>[2x]GSHMASMPKQLSSVTFHNGRKMPVVGLGTWQSPPEEVTAAIDVALEVGYRHIDTAFMYQNEAAIGKTLKKWFDSGKLKREDVFIVTKLPPIGNRAESVEKFLTKSLEALQLDYVDLYLIHLPVGFQYKGDDNLWPRGEAGEFLIDTSTDLISLWKAMEAQVDAGRTRSVGLSNFNSRQIARIVKSARIRPANLQVELNV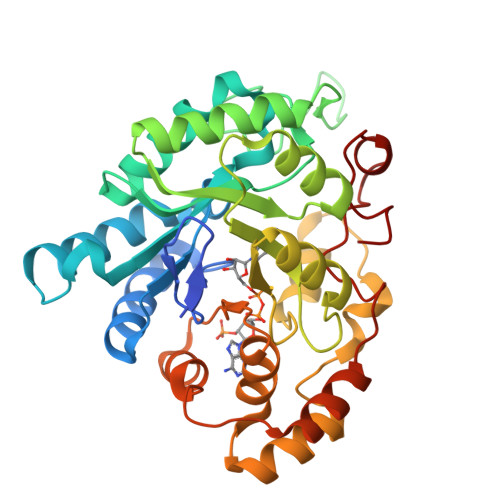YFQQRELVAFCRALDITVCAYAPIGSPGLANVIKARGAEVPESAKFDPLTDPVVLKIAEHHKKTPAQVLLRHCMQRDIVVIPKSTNAGRIKENFQVFDFELSKAEVDELDSLDKRAAGRRFRMDQYKGLREHPEHPYDEPY>[4x]MVQKWMQRMIIVDNNKLNVRALPSFIDYFNGIYGFATGIKDIMGMIFKTDTGGSNLTLDEILKNQNLLNDISGKLDGINGDLGDLIAQGNLNSELAKELLKISNEQNQMLNHVNAQLNAINSTLNIYLPKITSMLNEVMKQNHVLSLQIEFLSKQLQEISDKLDIINLNVLINSTLTEITPAYQRIKYVNEKFDELTSTVEKNPKSYQDNVTKEVIENLNELTELAKSVTKNDMDSFEFYLQTFHDVMTGNNLFGRSALKTASELITKENVTTRGSEIGKVYNFLIVLTSLQAKAFLTLTACRKLLGLTDIDYTQIMNHHIDGQKREFRINILPTLSNNFSNPSYSKNRGSDIDDPIV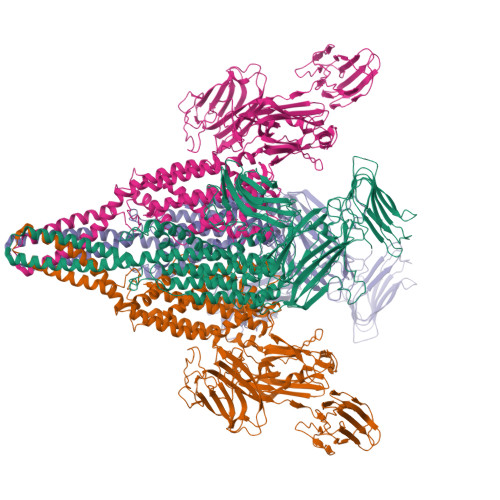VLEAAPGYALIGFEILNDPLPILKGYQARLKPNYQVDRESMSETIYGDIHKLFCPKQLEQKYYIKDIEFPEGYVITKIVFEKRLNQLGYEVTANFYDPSTGSIDLNKVKVESWKEKSCEEDSCEDEYSIIKAETDGIYMPLGVVSETFLTPIYGFGLTVDEKNQKITLTGKSYLRESLLETDLLNNETYLIASPDGYISSIVENWNITSDNTGSWRANNNNAFVDKADTIKGSSSLYTHKDGEFSQFIGNKLKPKTNYVIQYVIKGRPAIYLKNNKDTLFEDTKNNFSDFQTVTKKFNSGVNPSEIYFLFKNQSEYEAWGNNFIILEIKSLEFLPQMLKPEDWIPSGNVQMKDGGRLEILGDGYFKQFIKLENDSTYHLRLSVKGTGRVSIIDESKYLLFVNVKDEDLTRVIKNTSSKGECFIALEGTYVENSSTIFSNVSIVKE> MIHELLLALSGYPGSIFTWNKRGGLQVSQDFPFLHPSETSVLNRLCRLGTDYIRFTEFIEQYTGHVQQQDHHPSQQGQGGLHGIYLRAFCTGLDSVLQPYRQALLDLEQEFLADPHLSISHINYSLD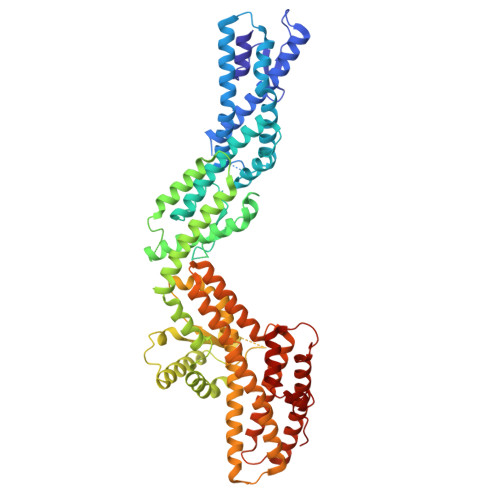QFQLLFPSVMVVVEQIKSQKIHGCQILETVYKHSCGGLPPVRSALEKILAVCHGVMYKQLSAWMLHGLLLDQHEEFFIKQGPSSGNVSAQPEEDEEDLGIGGLTGKQLRELQDLRLIEEENMLAPSLKQFSLRVEILPSYIPVRVAEKILFVGESVQMFENQNVNLTRKGSILKDQEDTFAAELHRLKQQPLFSLVDFEQVVDRIRSTVAEHLWKLMVEESDLLGQLKIIKDFYLLGRGELFQAFIDTAQHMLKTPPTAVTEHDVNVAFQQSAHKVLLDDDNLLPLLHLTIEYHGKEHKADATQAREGPSRETSPREAPASGWAALGLSYKVQWPLHILFTPAVLEKYNVVFKYLLSVRRVQAELQHCWALQMQRKHLKSNQTDAVKWRLRNHMAFLVDNLQYYLQVDVLESQFSQLLHQINSTRDFESIRLAHDHFLSNLLAQSFILLKPVFHCLNEILDLCHSFCSLVSQNLGPLDERGAAQLSILVKGFSRQSSLLFKILSSVRNHQINSDLAQLLLRLDYNKYYTQAGGTLGSFGM> AIWELKKDVYVVELDWYPDAPGEMVVLTCDTPEEDGITWTLDQSSEVLGSGKTLTIQVKEFGDAGQYTCHKGGEVLSHSLLLLHKKEDGIWSTDILKDQKEPKNKTFLRCEAKNYSGRFTCWWLTTISTDLTFSVKSSRGSSDPQGVTCGAATLSAERVRGDNKEYEYSVECQEDSACPAAEESLPIEVMVDAVHKLKYENYTSSFFIRDIIKPDPPKNLQLKPLKNSRQVEVSWEYPDTWSTPHSYFSLTFCVQVQGKSKREKKDRVFTDKTSATVICRKNASISVRAQDRYYSSSWSEWASVPCS;> RAVPGGSSPAWTQCQQLSQKLCTLAWSAHPLVGHMDLREEGDEETTNDVPHIQCGDGCDPQGLRDNSQFCLQRIHQGLIFYEKLLGSDIFTGEPSLLPDSPVGQLHASLLGLSQLLQPEGHHWETQQIPSLSPSQPWQRLLLRFKILRSLQAFVAVAARVFAHGAATLSPHHHHHH;> GLRERCVRNY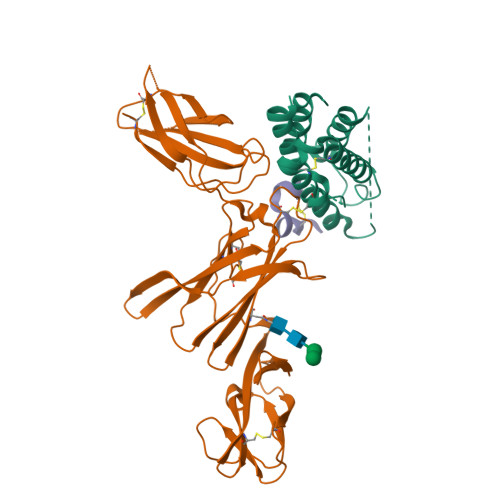GHEFCQNWYW> GAMGEQIFYWS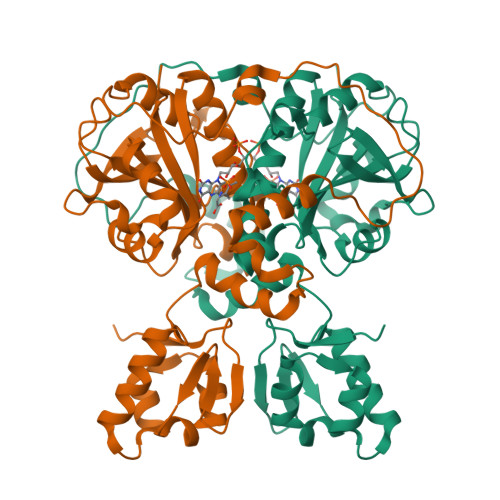PAKHWRMSDEGVVIGESTYTGMILEWFPEFYFFAQTGVTINRLLERFSSGSEKEANEILELLIQDRVLVEGILPPREVFSPQEGLFVNPYSEQIRYSKEALDYYVSEQLNRTHAACRSTKIQLETSGALPDIIQKRRSCRRFDMKTPVSFATFSNLLSSLKQRKEDKILYNYASAGGLYPIDVFVYVKPRRVEGVKAGFYYFNPADHSLVLVNNIDQVIKDDHELINQDIFAQSAFSVYLVYNARASMPKYGAAGYFYACIEAGIITATLNMVAEDLNVGLCSIGHMNFEEIQTFLKLEDHQVILHAIEGGLKIDGAAAENLYFQ N-(1,1-dioxo-1-thian-4-yl)-5-methyl-4-oxo-7-3-(trifluoromethyl)phenyl-4H,5H-thieno-3,2-c-pyridine-2-carboximidamide 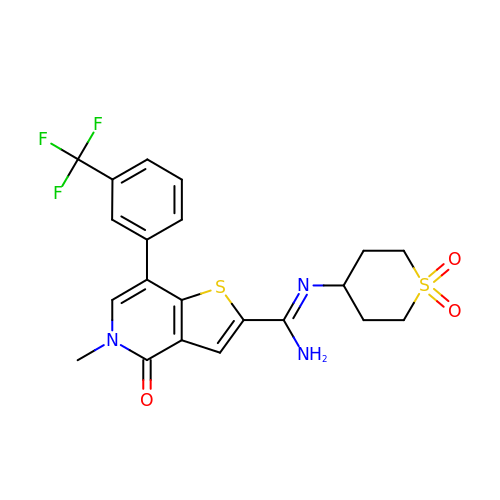| C21 H20 F3 N3 O3 S2 | UCISVEKCUIGBJX-UHFFFAOYSA-N> GASGSERLLDELTLEGVARYMQSERCRRVICLVGAGISTSAGIPDFRSPSTGLYDNLEKYHLPYPEAIFEISYFKKHPEPFFALAKELYPGQFKPTICHYFMRLLKDKGLLLRCYTQNIDTLERIAGLEQEDLVEAHGTFYTSHCVSASCRHEYPLSWMKEKIFSEVTPKCEDCQ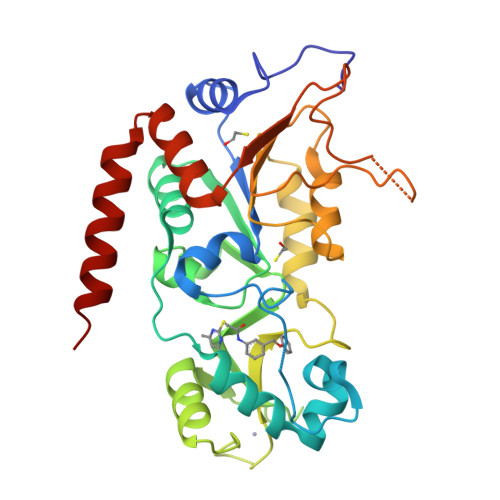SLVKPDIVFFGESLPARFFSCMQSDFLKVDLLLVMGTSLQVQPFASLISKAPLSTPRLLINKEKAGQSDPFLGMIMGLGGGMDFDSKKAYRDVAWLGECDQGCLALAELLGWKKELEDLVRREHASIDAQS> DYWRAKHHP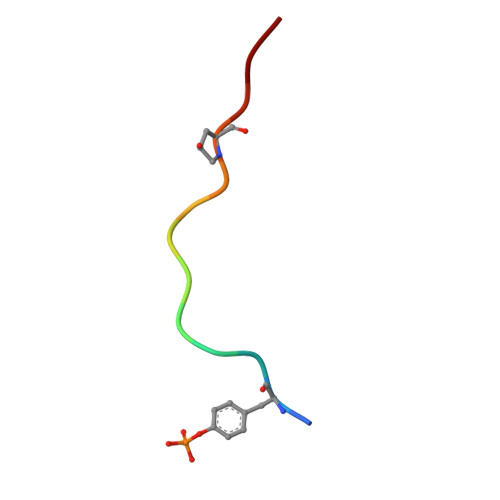PKNN> MANTPVNYQLTRTANAIPEIFVGGTFAEIKQNLIEWL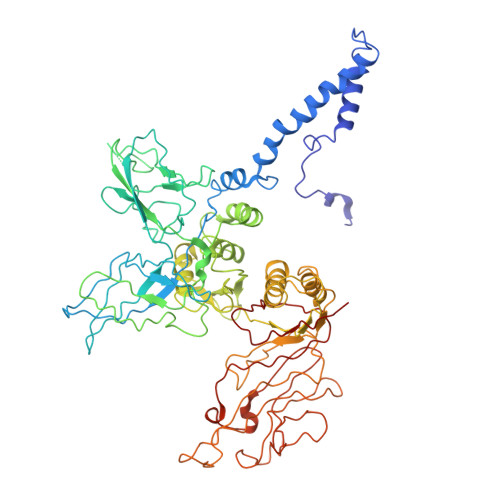NGQNEFLDYDFEGSRLNVLCDLLAYNTLYIQQFGNAAVYESFMRTANLRSSVVQAAQDNGYLPTSKSAAQTEIMLTCTDALNRNYITIPRGTRFLAYAKDTSVNPYNFVSREDVIAIRDKNNQYFPRLKLAQGRIVRTEIIYDKLTPIIIYDKNIDRNQVKLYVDGAEWINWTRKSMVHAGSTSTIYYMRETIDGNTEFYFGEGEISVNASEGALTANYIGGLKPTQNSTIVIEYISTNGADANGAVGFSYADTLTNITVININENPNDDPDFVGADGGGDPEDIERIRELGTIKRETQQRCVTATDYDTFVSERFGSIIQAVQTFTDSTKPGYAFIAAKPKSGLYLTTVQREDIKNYLKDYNLAPITPSIISPNYLFIKTNLKVTYALNKLQESEQWLEGQIIDKIDRYYTEDVEIFNSSFAKSKMLTYVDDADHSVIGSSATIQMVREVQNFYKTPEAGIKYNNQIKDRSMESNTFSFNSGRKVVNPDTGLEEDVLYDVRIVSTDRDSKGIGKVIIGPFASGDVTENENIQPYTGNDFNKLANSDGRDKYYVIGEINYPADVIYWNIAKINLTSEKFEVQTIELYSDPTDDVIFTRDGSLIVFENDLRPQYLTIDLEPISQ>MAENKLGRDIPRKYANQYGVFEGELAHIKSYKESSRQVKPVKPSDDKLLSSIHEAIEKTRLKDGMTISFHHHFREGDYVMNMVLDEIAKMGIKDISIAPSSIANVHEPLIDHIKNGVVTNITSSGLRDKVGAAISEGIMENPVIIRSHGGRARAIATDDIHIDVAFLGAPSSDAYGNANGTRGKTTCGSLGYAMIDAKYADQVVIVTDTLVPYPNTPISIPQTDVDYIVVVDAIGDPEGIAKGATRYTKNPKELLIAEYAAKVITSSPYYKEGFSFQTGTGGASLAVTRFMREQMIKDDIKANFALGGITNAMVELLEEGLVDKILDVQDFDHPSAVSLDRNAEKHYEIDANMYASPLSKGSVINQLDICVLSALEVDTNFNVNVMTGSDGVIRGASGGHCDTAFAAKMSLVISPLVRGRIPTFVDKVNTVITPGTSVDVVVTEVGIAINPNRPDLIEYFKDLKVPQLTIEELKEKAYAIVGNPQPIQYGDKIVALIEYRDGSLIDVVRNVLEH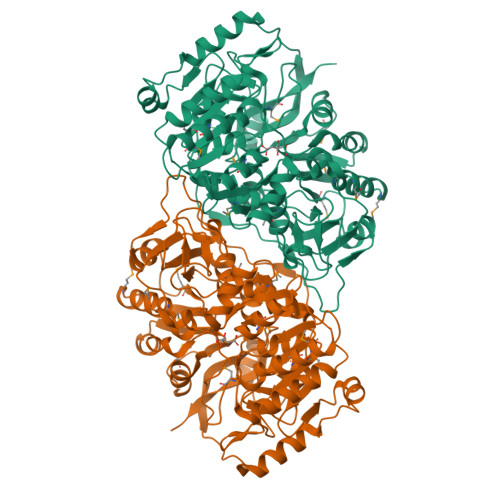HHHHH[2x]ticlopidine | C14 H14 Cl 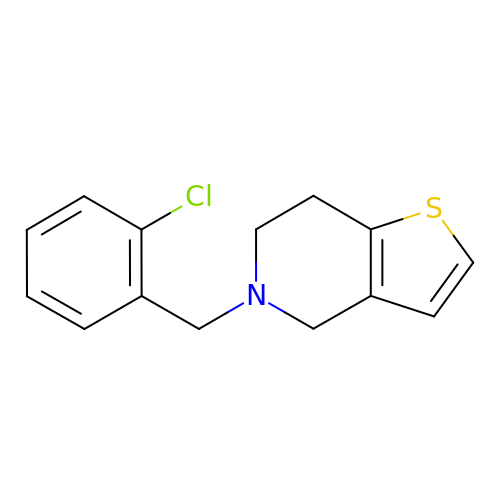N S | PHWBOXQYWZNQIN-UHFFFAOYSA-N> KAL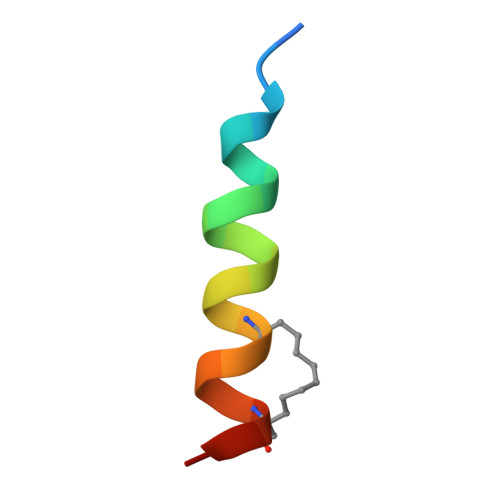ETLRRVGDGVLRNHLTAF>SNMKKNQPNVVLIVVDQMRADALSLNSQDKIISTPTLDMMASQGYNFENCYSPVPSCVPARAALLTGLDQETSGRVGYEDEVPWNFKNTLPEVFKEQGYQTECIGKMHVYPSRKRLGFDHVLLHDGYLHVDRKYDKSYGEQFEYSSDYLMFLKESLGSDADLIDDGLNCNSWEARPWMYPEKFHPTNWVVSEGINFLRRKDPTVPFFLKLSFEKPHAPLNPPKYYFDMYMDRLPDTLDLHIGNWEKLEHVVPDVCALRGRLKEDDQRRMLAGYYGLISHIDHQINRFLMALKEFRHDKDTIIWFISDHGDQLGEHYLFRKGYPYQGSIRIPSFIYDPGDLISAKKHGIKELVKIQDIFPSLVDLVLGQYVNTDGKSVKQLLFGNCEGWRREIHGEHSLGLDSSQYILTEKWKFIWFPVKNTYQLFDMINDPNEMKNLYYDKKYESIIYEMKHKLVGYLKGREEGFVKNGQLIQIGISNIVSTLKSKK[2x]

In this study, we determined the crystal structure of an arylsulfatase from Enterococcus faecium (EfAS), revealing a homotetrameric assembly with a windmill-like architecture not observed in other known arylsulfatases or phosphonoester hydrolases. Arylsulfatases, a subset of sulfatases, catalyze the hydrolysis of aryl sulfate esters to produce aryl compounds and inorganic sulfate. Functional assays and site-directed mutagenesis showed that EfAS hydrolyzes sulfates, phosphates, and phosphonates, indicating broad substrate specificity. Furthermore, high-performance liquid chromatography–mass spectrometry demonstrated that EfAS removes sulfate groups from key bioactive molecules, such as caerulein and estrone sulfate.

The crystal structure of EfAS was determined at 1.96  Å resolution in the P4212 space group, with two crystallographically independent molecules in the asymmetric unit. Structural analysis revealed that EfAS forms a homotetramer through symmetry-related operations, comprising four identical subunits arranged around a central fourfold rotational axis—resembling a windmill assembly. The formation of the homotetramer is primarily mediated by interactions between loops and α-helices of adjacent subunits, involving multiple hydrogen bonds, salt bridges, and hydrophobic interactions. The catalytic center of EfAS is located within a groove on the protein’s surface, positioned near the interface between two adjacent subunits. EfAS exhibits a characteristic AP superfamily α/β-fold structure, featuring two β-sheet domains: an N-terminal six-stranded (β1–β6) and a C-terminal four-stranded (β7–β10) β-sheet, encompassed by ten α-helices (α1–α10). In our crystal structure, C61 displays dual conformations: unmodified C61 with its –SH group coordinating Mn²+, and HFG61 covalently bound to sulfate, forming a sulfate-ester intermediate (FGS), likely resulting from crystallization in the presence of p-nitrophenyl sulfate. Metal coordination analysis revealed that optimal electron density maps and B-factors were observed exclusively with Mn²+, not Ca²+ or Mg²+, which correlates with subsequent activity assays showing Mn²+-specific catalysis. Structural analysis reveals distinctive features of EfAS within the AS/PMH superfamily. While the active site maintains core features of divalent metal coordination through two aspartates (D20 and D311) and the catalytic cysteine (C61), EfAS shares the distinctive fourth coordinating histidine (H312) with PMHs and SpAS2, diverging from the asparagine found in classical ASs (Fig. 4A through G). The substrate-binding pocket of EfAS exhibits an elongated and narrow shape, delineated by residues S60, Y82, L132, H133, N174, R323, and K324, which form the outer boundary of the pocket.>MMGPVWRKHYITYRINNYTPDMNREDVDYAIRKAFQVWSNVTPLKFSKINTGMADILVVFARGAHGDDHAFDGKGGILAHAFGPGSGIGGDAHFDEDEFWTTHSGGTNLFLTAVHEIGHSLGLGHSSDPKAVMFPTYKYVDINTFRLSAD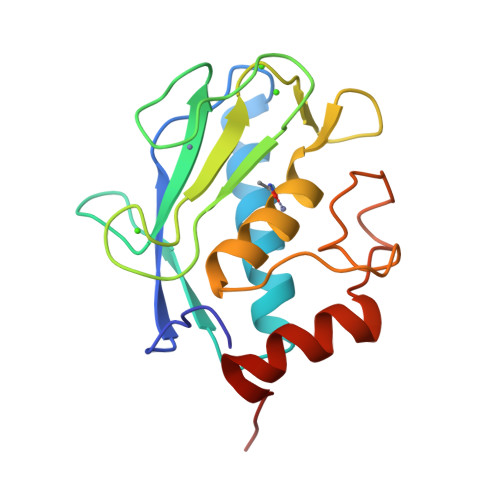DIRGIQSLYGDPKEN[6x]> 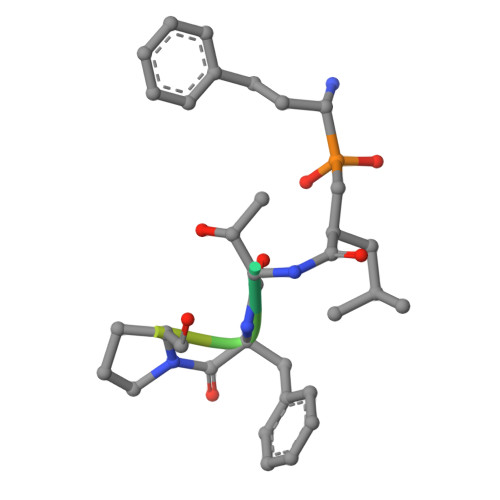XXTFPETLTY> SLIISERKEEGETVTWDLSLSEDSNENEKKAWKRYFERYGLTDEEISKIESIRVEGTEEEVEKMYYYYKLELEIREKLNSEETEEKLEEIWRLSSKGTEENLKEAKEIIKELLKEIGYKE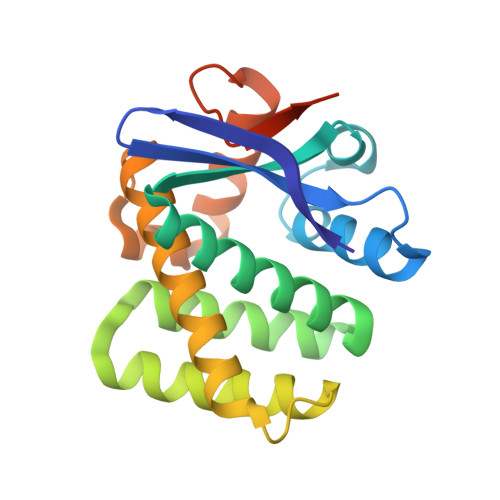DVEKKAEEYLEGLQKYLDYLSKKFGITREQLGKRETRSKLYRESLENPEKYPLFKLKGGSGGSHHHHHH To prevent cell suicide, A. radiobacter K84 contains a second, non-essential LeuRS, termed AgnB2, which is resistant to TM84. The aminoacylation of tRNALeu is catalysed in a two-step mechanism in all LeuRSs: in the tRNA-independent first step, leucine is activated by ATP to form the essential obligate intermediate leucyl-adenylate (Leu-AMP) that is stably bound to the enzyme. In the second step, a bound tRNALeu repositions its CCA 3′-end into the LeuRS active site where activated-leucine is transferred to the tRNA. TM84 (agrocin 84) is a highly potent LeuRS toxin that employs a unique tRNA-dependent inhibition mechanism.

We obtained an X-ray crystal structure of AgnB2 in complex with tRNALeu and Leu-AMS; the final model was refined to a final R-factor of 19.4% (R-free=23.8%) and a final resolution of 2.1 Å. In the case of AgnB2, the highly conserved methionine of the KMSKS motif is interestingly replaced by a glutamine residue (Q573). Our structure shows that Leu-AMS is bound in the active site with the mobile KQSKS loop present in a semi-open conformation. The equivalent position in AgnB2, Q573, forms a hydrogen bond side-chain interaction with the side chain of T581, which is found to be a conserved hydrophobic residue in TM84 sensitive LeuRSs (I628 in LeuRSEc). Importantly, the presence of A102 in AgnB2, instead of an asparagine as found in the LeuRSEc structure (N104), leads to loss of an H-bond interaction between the α-helix (96–114) and a main-chain peptide bond located at T42 (P45 LeuRSEc). The missing LS-domain in AgnB2 is replaced by a small connecting loop that contains a salt bridge between residues D567 and R571. Importantly, the AgnB2 structure shows the equivalent residue to R418 in LeuRSEc is the neutrally charged Q413.

>MQYDHRSRDAFWQQKWDEKRIFDWDPSSPGKKFYVLEMFPYTSGHLHIGHVRNYSMGDTLARMQIARGYSVLHPMGWDSFGLPAENAARKFGTHPAKFTQDAIDSMKRSMMQLGFGYSWANELATCSPTYVLAQQKLFLDLYRKGLIYRDDTYVYWDPVEQTVLAAEQVIDGKGWRSGAAVYKRRTPQWFVDIRSYADRLLDDLESLEGWPTSVRNIQRNWIGRTEGAEVRFLVEASDLTINAFTTRLDTLAGCTFIALAPEHTILDELPIPSQMRASVKDYCESILVLSSEERSAGAKSGIFTGLMVVNPLNQERVPLYVANYVMPDFGTGAVIGVPAHDERDADFGALFGLPVRVVISTDSDATGLNIADGIVTNSHSLVDGLTSSAAREILIAHLSEKLEGQKSTQYRLQNWSISRQRYWGCPIPIIHCSECGTIPVAEEQLPILLPDHLISEGSGSPLSRDESWMKAKCPQCGGDAARDPDTMDTFVDSSWYFLRYPSPSSPNPIDSSLCNKIAPADVYIGGIEHATLHLIYSRFITKVLHDLGYIEFDEPFVELYNQGMVNDVHGRKQSKSLGNVTDPSVVVQEFGADAVRCYLLFKTTYNAPINWEDSGPQAMRSYLERVCRLFTNNLDRLRSSSAIEICPDDCENEEDREIARQLQLAIGKVTADVERFHFNAAIAAIMSVTNLLYEKGGKASPTVLAGSLRLLVRLLAPFAPHISEELWALSGCNSLVAAEPWPTINERLVQAENIVLPVQINGKLIRTMTIPVNLAEEDILSTVLALPEVRSRLSDRDLKNYRYVPNRIINLVVGLEHHHHHH[2x]> GSHMFTGLNTPSGVAVDSAGTVWVTDHGNNRVVKLAA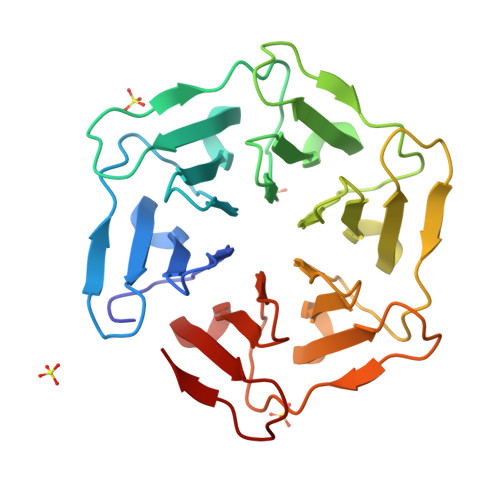GSNTQTVLPFTGLNTPSGVAVDSAGTVWVTDHGNNRVVKLAAGSNTQTVLPFTGLNTPSGVAVDSAGTVWVTDHGNNRVVKLAAGSNTQTVLPFTGLNTPSGVAVDSAGTVWVTDHGNNRVVKLAAGSNTQTVLPFTGLNTPSGVAVDSAGTVWVTDHGNNRVVKLAAGSNTQTVLPFTGLNTPSGVAVDSAGTVWVTDHGNNRVVKLAAGSNTQTVL We identify a horizontally transferred T6SS with Ntox15 family nuclease effector (Tde1) that mediates interbacterial antagonism among Bacteroidales, including several derived from a single human donor. Effectors with novel toxin 15 (Ntox15) DNAse domains, also known as toxin_43 domains, degrade recipient genomic DNA. Cognate immunity proteins are encoded adjacent to T6SS effectors and neutralize their activity to prevent intoxication of self and kin. Crystallographic snapshots of isolated Tde1, the Tde1/Tdi1 complex, and homologs from Phocaeicola vulgatus (Tde2/Tdi2) illustrate a conserved mechanism of immunity inserting into the central core of Tde, splitting the nuclease fold into two subdomains.

Tde1tox interaction with Tdi1 increases thermal stability (melting temperature 67°C versus 55.5°C). A Tde1tox/Tdi1 dissociation constant of 18 nM was measured by biolayer interferometry (BLI). We therefore obtained crystal structures of the Tde1 Ntox15 domain in complex with Tdi1, as well as a homologous complex from P. vulgatus dnLKV7, Tde2tox and Tdi2. The Tdetox/Tdi complex homologs exhibit very similar structure despite 51% sequence identity between the Ntox15 domains, indicating a conserved mode of effector–immunity interaction. When bound to immunity proteins, Tde1tox and Tde2tox split into two subdomains. There is an ~32 amino acid region disordered in the crystal structure, corresponding to β2, α6, and the surrounding loops in the Tde1tox only structure. Notably, this disordered region contains part of the HxxD active site motif and most of the DNA binding site. Superposition of the Tde1tox alone structure with the Tde1tox/Tdi1 complex indicates a conformational shift characterized by a hinge motion, as well as an ~180° relative rotation of the two Tde1tox subdomains. Upon immunity interaction, Tde effectors undergo a dramatic conformational shift, highlighted by superposition of the Tde1tox alone and Tde1tox/Tdi1 complex structures. The immunity protein does not sterically occlude the active site, but rather splits the effector into subdomains and structurally distorts the active site, which is disordered in the crystal structures.

>MHHHHHHSNKKSLSVIFVKPPFQLKKKFQKDPFYEIEMRKQLQMQQDGINNMTIFEWLKNRENFKKYGRNPKSKKIQEDFRDRYRNAKIDEYLLLYEDMDIKAIEAMVDSELEGLAALANPAQIAGGYVDVVTQMGNKRINSSIGSQWGSIEKGRSLNIENELLKLITDPPPITEEEQKKIKMNVNLVENLEIVK[2x];>[2x]MFEKFLERSGNSIKLEEFSEDYIRQYNNLVSEKLISFWRIAGIGIYCNGLFRTIIPNDYQYIIEECYPMYDYETVTPFMITVFGDIFAYVKNHVIGDYVVFINIRYGTFKILSENIDILLNIVIFNKSCLENWFLLNEYNTIKEVKAMPKIDECYGYVPALVAGGKDCIDNIQIVKIAPYIDTVIQLMGDLKRIR> MNFKVSQVEKLKWKIKCFENKFLNYRLSTNETAVAETEYGKVKGIKRLTVYDDSYYSFEGIPYAQPPLGELRFKAPQRPTPWDGVRDCCNNKDKSVQVDFITGKTCGSEDCLYLSVYTNNLAPETKRPVLVYIHGGGFVIGENHREYYGPDYFIKKDVVLITIQYRLGVLGFLSLNSEELNVPGNAGLKDQVMALRWIKNNCANFGGNPDNITVFGESAGGASAHYMMLTEQTRGLFHRGILMSGNAVCPWAISQNQHRAYAIAKLNGYKGENNDKDVLEFLMKAKAHDLIKLEDKVLTPEEHVNKVMFAFGPTVEPYQTADCV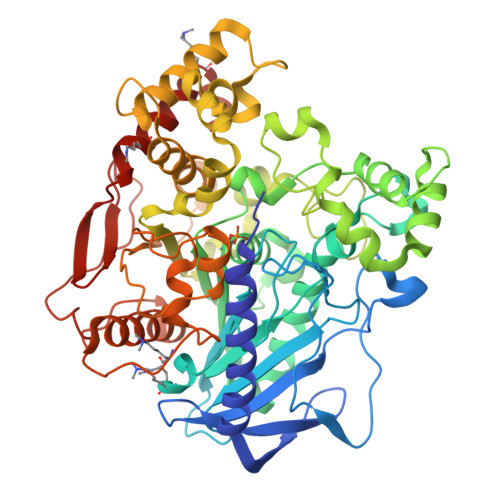LPKHPREMVKTAWGNSIPTMMGNTSYEGLLFTPIVKQMPALLKELETCANFVPTELADSERSSAETLELGAKIKKAHVTGETPTNDNFLDLCSHFYFWFPMHRLLQIRFKHTSGTPVYLYRFDFDSEEIINPYRIMRHGRGVKGVSHADELTYLFWNALAKRLPKESREYKTIERMVGIWTQFATTGNPYSNEIDGLENIIWDPIKKSDEVYKCLNISDELKIIDVPEMEKIKQWESLYEKRKDLF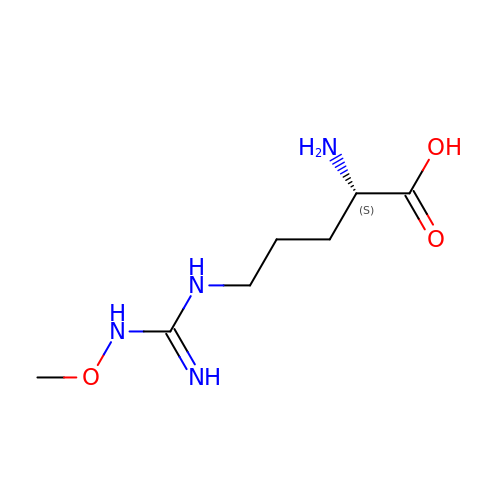N~5~-(N-methoxycarbamimidoyl)-L-ornithine | C7 H16 N4 O3 | FRTXFDDNHUEGNE-YFKPBYRVSA-N>[2x]MPVLENRAAQGDITAPGGARRLTGDQTAALRDSLSDKPAKNIILLIGDGMGDSEITAARNYAEGAGGFFKGIDALPLTGQYTHYALNKKTGKPDYVTDSAASATAWSTGVKTYNGALGVDIHEKDHPTILEMAKAAGLATGNVSTAELQDATPAALVAHVTSRKCYGPSATSEKCPGNALEKGGKGSITEQLLNARADVTLGGGAKTFAETATAGEWQGKTLREQ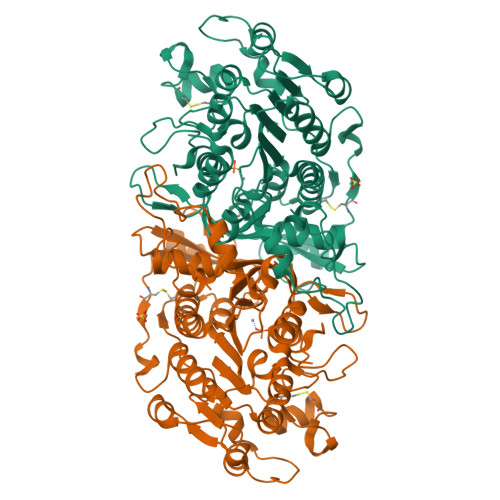AEARGYQLVSDAASLNSVTEANQQKPLLGLFADGNMPVRWLGPKATYHGNIDKPAVTCTPNPQRNDSVPTLAQMTDKAIELLSKNEKGFFLQVEGASIDKQDHAANPCGQIGETVDLDEAVQRALEFAKKEGNTLVIVTANHAHASQIVAPDTKAPGLTQALNTKDGAVMVMSYGNSEEDSQEHTGSQLRIAAYGPHAANVVGLTDQTDLFYTMKAALGLK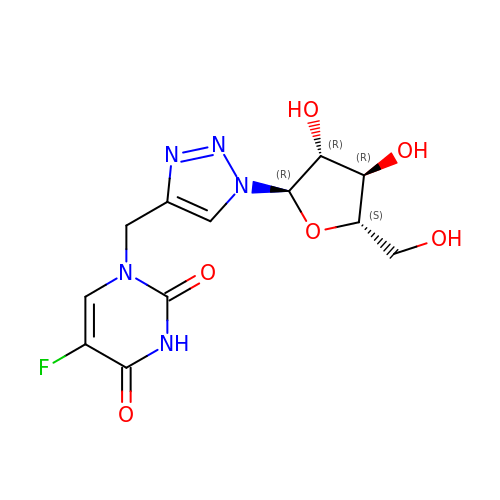1-{[1-(alpha-L-arabinofuranosyl)-1H-1,2,3-triazol-4-yl]methyl}-5-fluoro-2,4-dioxo-1,2,3,4-tetrahydropyrimidine | C12 H14 F N5 O6 | MGDQWTKSRPEJPQ-WYOJIJJFSA-N>AMAPAKKSEELVAEAHNLCTLLENAIQDTVREQDQSFTALDWSWLQTE[2x];>MWEQGAPETLQRCLEENQELRDAIRQSNQILRERCE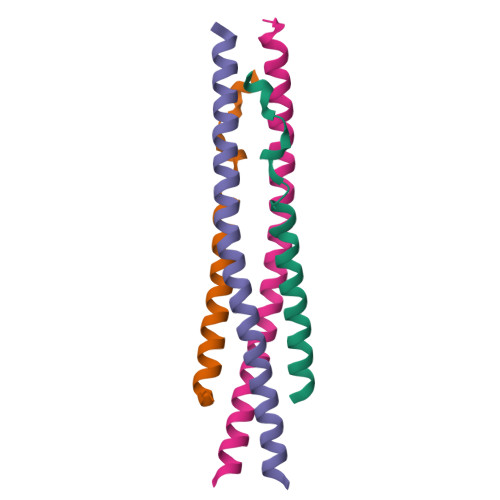ELLHFQASQREEKEFLMCKFQEARKLVERLGLEK[2x]CILASTATIN 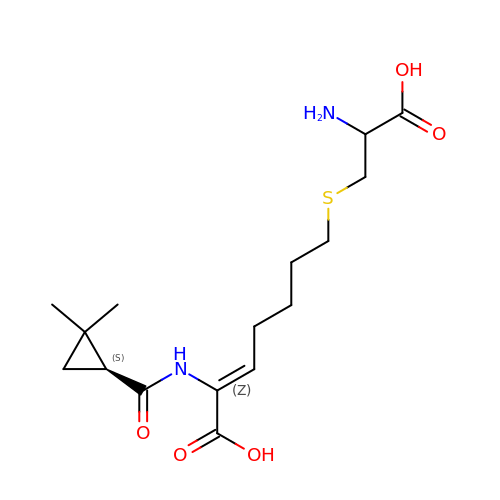| C16 H26 N2 O5 S | DHSUYTOATWAVLW-MSSAFCDDSA-N>SLLPKDISQLLSLVSATINGVDNPWSKDQISYFRTLLKVLFVVLRGTKHSNNAAPQKPTAESPVAVTQLVLTTLDRVVARSFRNLAALVHEPDAATTPEDLALITAILQACLSVPGIEQCQLQVLNIMSSHNVLQVATSLFSWSDRLAEKGDPIYGELALLLLLELSALPALAEQLACDGLLGHLTSANLAGFMRRANVSPFTDNAGAARCYAIWAKGILPLLLNILGALGATIAPEVAFVLNQFPNLLRSSVDRLEAPG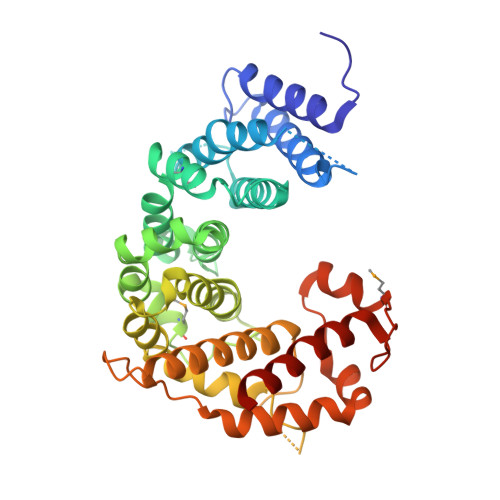LSRTVPLSSRDAPGAGPHYFVALVALSEVHSLALLTRVLAALRSGNARDIPEVVWDSGAVLENVEFWLASRKVLRERLLPLNPREAEWRGMKASEGSGCETKLEEKAVGLLEGIRDVLAEEEE[2x]> HKEAGQDVVTSNFDASKIAG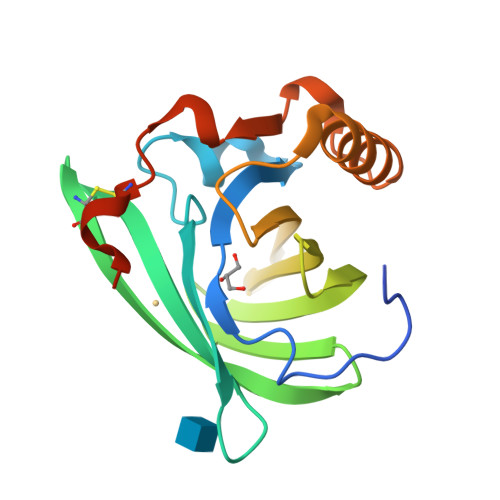EWYSILLASDAKENIEENGSMRVFVEHIRVLDNSSLAFKFQRKVNGECTDFYAVCDKVGDGVYTVAYYGENKFRLLEVNYSDYVILHLVDVNGDKTFQLMEFYGRKPDVEPKLKDKFVEICQQYGIIKENIIDLTKIDRCFQLRGSGGVQESSAE> MSGKDRIEIFPSRMAQTIMKARLKGAQTGRNLLKKKSDALTLRFRQILKKIIETKMLMGEVMREAAFSLAEAKFTAGDFSTTVIQNVNKAQVKIRAKKDNVAGVTLPVFEHYHEGTDSYELTGLARGGEQLAKLKRNYAKAVELLVELASLQTSFVTLDEAIKITNRRVNAIEHVIIPRIERTLAYIITELDEREREEFYRLKKIQEKKKILKEKSDKDLEQRRAAGEVIEPANLLAEEKDEDLLFE;>[3x]MDFSKLPKIRDEDKESTFGYVHGVSGPVVTACDMAGAAMYELVRVGHSELVGEIIRLEGDMATIQVYEETSGVSVGDPVLRTGKPLSVELGPGIMGAIFDGIQRPLSDISSQTQSIYIPRGVNVSALSRDVKWDFTPCKNLRVGSHITGGDIYGIVNENSLIKHKIMLPPRNRGTVTYIAPPGNYDTSDVVLELEFEGIKEKFSMVQVWPVRQVRPVTEKLPANHPLLTGQRVLDALFPCVQGGTTAIPGAFGCGKTVISQSLSKYSNSDVIIYVGCGERGNEMSEVLRDFPELTMEVDGKVESIMKRTALVANTSNMPVAAREASIYTGITLSEYFRDMGYHVSMMADSTSRWAEALREISGRLAEMPADSGYPAYLGARLASFYERAGRVKCLGNPEREGSVSIVGAVSPPGGDFSDPVTSATLGIVQVFWGLDKKLAQRKHFPSVNWLISYSKYMRALDEYYDKHFTEFVPLRTKAKEILQEEEDLAEIVQLVGKASLAETDKITLEVAKLIKDDFLQQNGYTPYDRFCPFYKTVGMLSNMIAFYDMARRAVETTAQSDNKITWSIIREHMGEILYKLSSMKFKDPVKDGEAKIKADYAQLLEDMQNAFRSLED;>[3x]MALRAMRGIVNGAAPELPVPTSGPLAGSREQALAVSRNYLSQPRLTYKTVSGVNGPLVILDHVKFPRYAEIVHLTLPDGTKRSGQVLEVSGSKAVVQVFEGTSGIDAKKTSCEFTGDILRTPVSEDMLGRVFNGSGKPIDRGPVVLAEDFLDIMGQPINPQCRIYPEEMIQTGISAIDGMNSIARGQKIPIFSAAGLPHNEIAAQICRQAGLVKKSKDVVDYSEENFAIVFAAMGVNMETARFFKSDFEENGSMDNVCLFLNLANDPTIERIITPRLALTTAEFLAYQCEKHVLVILTDMSSYAEALREVSAAREEVPGRRGFPGYMYTDLATIYERAGRVEGRNGSITQIPILTMPNDDITHPIPDLTGYITEGQIYVDRQLHNRQIYPPINVLPSLSRLMKSAIGEGMTRKDHADVSNQLYACYAIGKDVQAMKAVVGEEALTSDDLLYLEFLQKFERNFIAQGPYENRTVYETLDIGWQLLRIFPKEMLKRIPQSTLSEFYPRDSAKH;> MGHHHHHHGNSRSRVGRSFCSQFLPEEQAEIDQLFDALSSDKNSPNVSSKSFSLKALQNHVGEALPPEMVTRLYDGMRRVDLTGKAKGPSENVSQEQFTASMSHLLKGNSEEKSLMIMKMISATEGPVKAREVQKFTEDLVGSVVHVLSHRQELRGWTGKEAPGPNPRVQVLAAQLLSDMKLQDGKRLLGPQWLDYDCDRAVIEDWVFRVPHVAIFLSVVICKGFLVLCSSLDLTTLVPERQVDQGRGFESILDVLSVMYINAQLPREQRHRWRLLFSSELHGHSFSQLCGHITHRGPCVAVLEDHDKHVFGGFASCSWEVKPQFQGDNRCFLFSICPSMAVYTHTGYNDHYMYLNHGQQTIPNGLGMGGQHNYFGLWVDVDFGKGHSRAKPTCTTYNSPQLSAQENFQFDKMEVWAVGDPSEEQLAKGNKSILDADPEAQALLEISGHSRHSEGLRE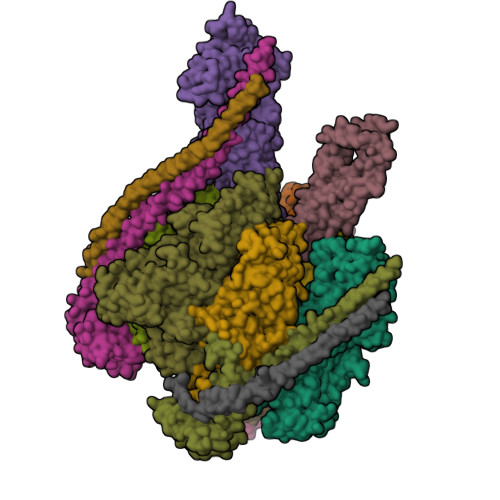VPDDE;>[3x]MALSDADVQKQIKHMMAFIEQEANEKAEEIDAKAEEEFNIEKGRLVQTQRLKIMEYYEKKEKQIEQQKKIQMSNLMNQARLKVLRARDDLITDLLNEAKQRLSKVVKDTTRYQVLLDGLVLQGLYQLLEPRMIVRCRKQDFPLVKAAVQKAIPVYKVATKRDVDVQIDQEAYLPEEIAGGVEIYNGDRKIKVSNTLESRLDLIAQQMMPEVRGALFGANANRKFLD;>MASQSQGIQQLLQAEKRAAEKVADARKRKARRLKQAKEEAQMEVDQYRREREQEFQSKQQAAMGSQGNLSAEVEQATRRQVQGMQSSQQRNRERVLAQLLGMVCDVRPQVHPNYRIAA[3x]> MGLLLLVLILTPSLAAYRHPDFPLLEKAQQLLQSTGSPYSTNCWLCTSSSTETPGTAYPASPREWTSIEAELHISYRWDPNLKGLMRPANSLLSTVKQDFPDIRQKPPIFGPIFTNINLMGIAPICVTAKRKNGTNVGTLPSTVCNVTFTVDPNQQTYQTYTHNQFRHQPRFPKPPNITFPQGTLLDKSTRFCQGRPSSCSTRNFWFRPADYNQCLQISNLSSTAEWVLLDQTRNSLFWENKTKGANQSQTPCVQVLAGMTIATSYLGISAVSEFFGTSLTPLFHFHISTCLKTQGAFYICGQSIHQCLPSNWTGTCTIGYVTPDIFIAPGNLSLPIPIYGNSPLPRVRRAIHFIPLLAGLGILAGTGTGIAGITKASLTYSQLSKEIANNIDTMAKALTTMQEQIDSLAAVVLQNRRGLDMLTAAQGGICLALDEKCCFWVNQSGKVQDNIRQLLNQASSLRERATQGWLNWEGTWKWFSWVLPFIGPLVSLLLLLLFGPCLLNLITQFVSSRLQAIKLQTNLSAGRHPRNIQESPF;> MAKGEGAESGSAAGLLPTSILQSTERPAQVKKEPKKKKQQLSICNKLCYAVGGAPYQVTGCALGFFLQIYLLDVAQVGPFSASIILFVGRAWDAITDPLVGFCISKSSWTRLGRLMPWIIFSTPLAVIAYFLIWFVPDFPHGQTYWYLLFYCLFETLVTCFHVPYSALTMFISTEQSERDSATAYRMTVEVLGTVLGTAIQGQIVGQADTPCFQDLNSSTVASQSANHTHGTTSHRETQNAYLLAAGVIA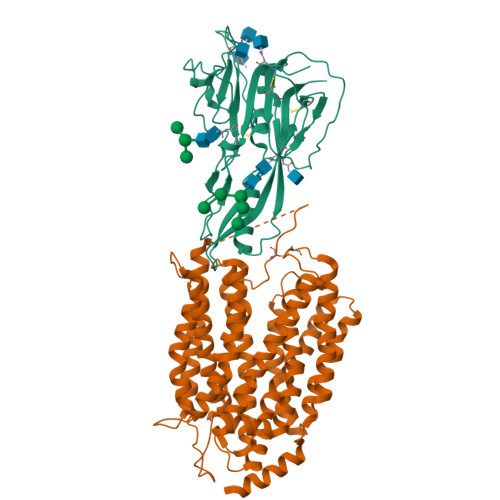SIYVICAVILTLGVREQREPYEAQQSEPMSFFRGLRLVMSHGPYIKLIAGFLFTSLAFMLVEGNFALFCTYTLGFRNEFQNLLLAIMLSATLTIPIWQWFLTRFGKKTAVYVGISSAVPFLILVALMESNLIVTYVVAVAAGISVAAAFLLPWSMLPDVIDDFHLKQPHSHGTEPIFFSFYVFFTKFASGVSLGISTLSLDFAGYQTRGCSQPERVKFTLKMLVTMAPIVLILLGLLLFKLYPIDEERRRQNKKALQALRDEASSSGCSETDSTELASIL>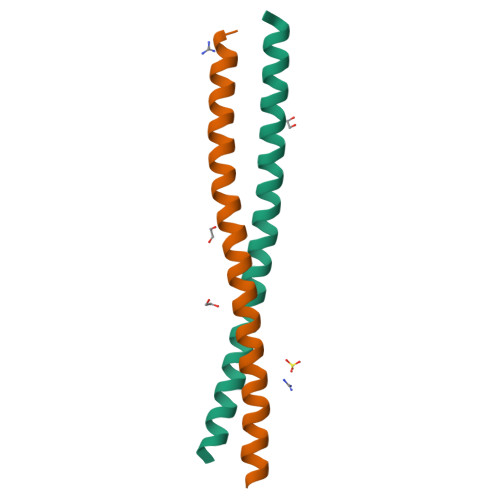[3x]GAMDPEFTKNALNVVKNDLIAKVDQLSGEQEVLRGELEAAKQAKVKLENRIKELEEELKRV> SGIVPQLQNIVSTVNLGCKLDLKTIALRARNAEYNPKRFAAVIMRIREPRTTALIFSSGKMVCTGAKSEEQSRLAARKYARVVQKLGFPAKFLDFKIQNMVGSCDVKFPIRLEGLVLTHQQFSSYEPELFPGLIYRMIKPRIVLLIFV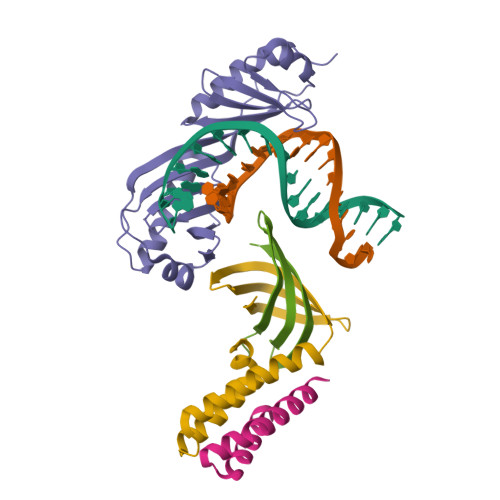SGKVVLTGAKVRAEIYEAFENIYPILKGFRKTT;> ANSANTNTVPKLYRSVIEDVINDVRDIFLDDGVDEQVLMELKTLWENKLMQSRAVDG;> GSGAEDGQVEEEPLNSEDDVSDEEGQELFDTENVVVCQYDKIHRSKNKWKFHLKDGIMNLNGRDYIFSKAIGDAEW;> AYQLYRNTTLGNSLQESLDELIQSQQITPQLALQVLLQFDKAINAALAQRVRNRVNFRGSLNTYRFCDNVWTFVLNDVEFREVTELIKVDKVKIVACDGKNTGSNTTE> MATGDERFYAEHLMPTLQGLLDPESAHRLAVRFTSLGLLPRARFQDSDMLEVRVLGHKFRNPVGIAAGFDKHG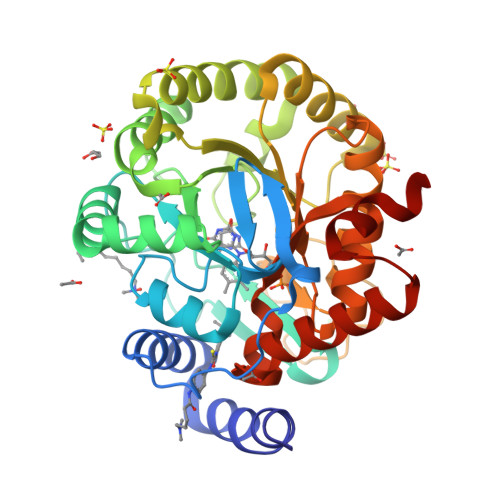EAVDGLYKMGFGFVEIGSVTPKPQEGNPRPRVFRLPEDQAVINRYGFNSHGLSVVEHRLRARQQKQAKLTEDGLPLGVNLGKNKTSVDAAEDYAEGVRVLGPLADYLVVNVSSPNTAGLRSLQGKAELRRLLTKVLQERDGLRRVHRPAVLVKIAPDLTSQDKEDIASVVKELGIDGLIVTNTTVSRPAGLQGALRSETGGLSGKPLRDLSTQTIREMYALTQGRVPIIGVGGVSSGQDALEKIRAGASLVQLYTALTFWGPPVVGKVKRELEALLKEQGFGGVTDAIGADHRR>[2x]GMAPPSVFAEVPQAQPVLVFKLIADFREDPDPRKVNLGVGAYRTDDCQPWVLPVVRKVEQRIANNSSLNHEYLPILGLAEFRTCASRLALGDDSPALQEKRVGGVQSLGGTGALRIGAEFLARWYNGTNNKDTPVYVSSPTWENLNGVFTTAGFKDIRSYRYWDTEKRGLDLQGFLSDLENAPEFSIFVLH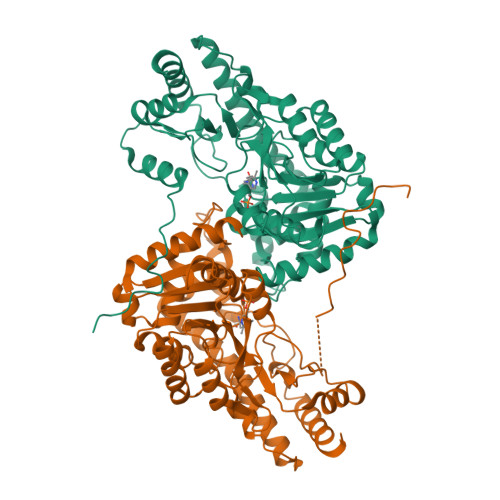ACAHNPTGTDPTPEQWKQIASVMKRRFLFPFFDSAYQGFASGNLEKDAWAIRYFVSEGFELFCAQSFSKNFGLYNERVGNLTVVAKEPDSILRVLSQMQKIVRVTWSNPPAQGARIVARTLSDPELFHEWTGNVKTMADRILSMRSELRARLEALKTPGTWNHITDQIGMFSFTGLNPKQVEYLINQKHIYLLPSGRINMCGLTTKNLDYVATSIHEAVTKIQ> SAHNAYNAGIMQKTGKAFADEFFAEENQVVAESNAVVLVLMKSDEIDAIIEDIVLKGGKAKNPSIVVEDKAGFW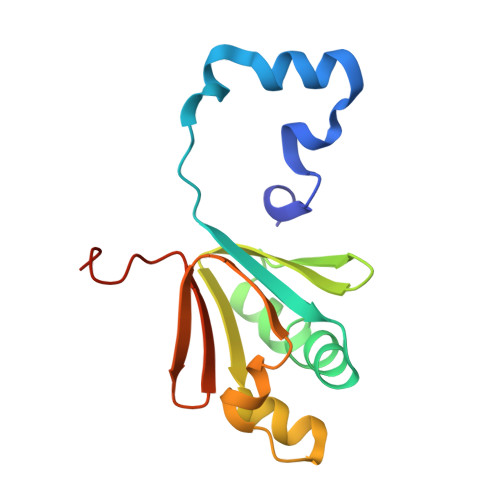WIKADGAIEIDAAEAGELLGKPFSVYDLLINVSSTVGRAYTLGTKFTITSELMGLDRALTDI(3R)-4-[(3R)-3-AMINO-4-(2,4,5-TRIFLUOROPHENYL)BUTANOYL]-3-(2,2,2-TRIFLUOROETHYL)-1,4-DIAZEPAN-2-ONE | C17 H19 F6 N3 O2 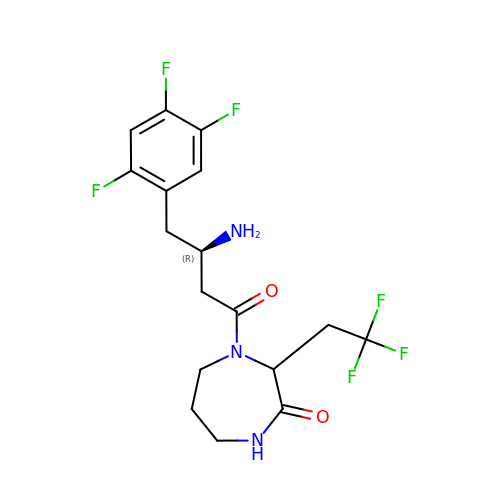| RMDAPSXWBVPVOG-IAPIXIRKSA-N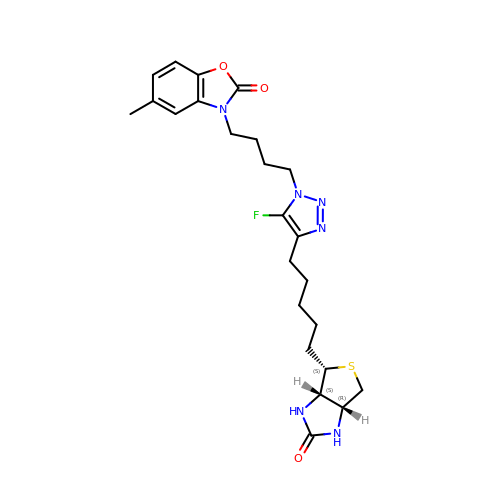3-[4-(5-fluoro-4-{5-[(3aS,4S,6aR)-2-oxohexahydro-1H-thieno[3,4-d]imidazol-4-yl]pentyl}-1H-1,2,3-triazol-1-yl)butyl]-5-methyl-1,3-benzoxazol-2(3H)-one | C24 H31 F N6 O3 S | DLFQUZRTJJWUQY-YYWHXJBOSA-N> GPGSEFDPGLPSTEDVILKTEQVTKNIQELLRAAQEFKHDSFVPCSEKIHLAVTEMASLFPKRPAL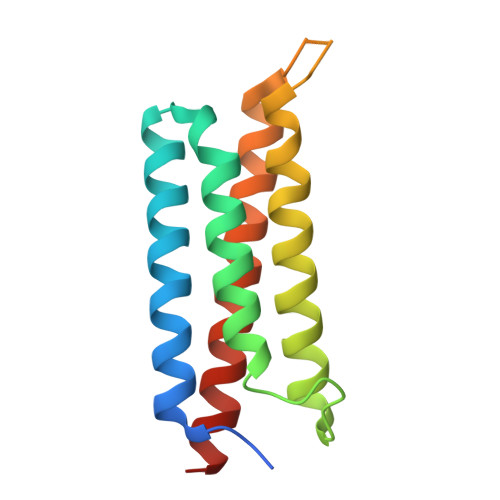EPVRSSLRLLNASAYRLQSECRKTVPPEPGAPVDFQLLTQQVIQCAYDIAKAAKQLVTITTREKKQ> MKKVVTVCPYCASGCKIN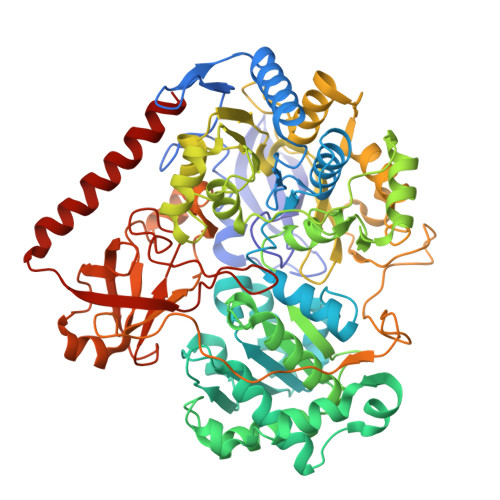LVVDNGKIVRAEAAQGKTNQGTLCLKGYYGWDFINDTQILTPRLKTPMIRRQRGGKLEPVSWDEALNYVAERLSAIKEKYGPDAIQTTGSSRGTGNETNYVMQKFARAVIGTNNVDCCARVUHGPSVAGLHQSVGNGAMSNAINEIDNTDLVFVFGYNPADSHPIVANHVINAKRNGAKIIVCDPRKIETARIADMHIALKNGSNIALLNAMGHVIIEENLYDKAFVASRTEGFEEYRKIVEGYTPESVEDITGVSASEIRQAARMYAQAKSAAILWGMGVTQFYQGVETVRSLTSLAMLTGNLGKPHAGVNPVRGQNNVQGACDMGALPDTYPGYQYVKDPANREKFAKAWGVESLPAHTGYRISELPHRAAHGEVRAAYIMGEDPLQTDAELSAVRKAFEDLELVIVQDIFMTKTASAADVILPSTSWGEHEGVFTAADRGFQRFFKAVEPKWDLKTDWQIISEIATRMGYPMHYNNTQEIWDELRHLCPDFYGATYEKMGELGFIQWPCRDTSDADQGTSYLFKEKFDTPNGLAQFFTCDWVAPIDKLTDEYPMVLSTVREVGHYSCRSMTGNCAALAALADEPGYAQINTEDAKRLGIEDEALVWVHSRKGKIITRAQVSDRPNKGAIYMTYQWWIGACNELVTENLSPITKTPEYKYCAVRVEPIADQRAAEQYVIDEYNKLKTRLREAALA(3-{[2-({N-[(2R)-2-hydroxy-3,3-dimethyl-4-(phosphonooxy)butanoyl]-beta-alanyl}amino)ethyl]sulfanyl}oxetan-3-yl)acetic acid | C16 H29 N2 O10 P S | 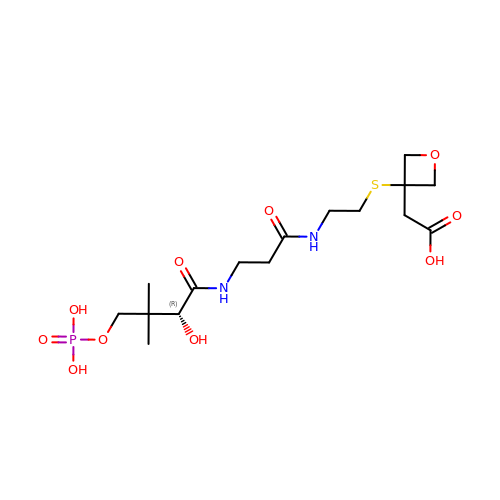WYVQKYVITQEIME-ZDUSSCGKSA-N The HNV F protein is a trimeric type I fusion protein that is initially expressed as an F precursor (F0), consisting of three domains (DI, DII and DIII), a C-terminal stem, a transmembrane domain and a cytoplasmic tail. We found that LayV F and MojV F both adopt a “tree-like” prefusion F structure similar to that of NiV, despite only sharing ~40% sequence conservation at the amino acid level. We show that despite sequence divergence from NiV, the F proteins adopt an overall similar structure but are antigenically distinct as they do not react to known antibodies or sera.

In August 2022, a novel henipavirus (HNV) named Langya virus (LayV) was isolated from patients with severe pneumonic disease in China. Based on the sequence of LayV, published in August 2022, we expressed the F ectodomain residues 1-478 without any heterologous stabilizing mutations. Through iterative particle picking, 2D classification and 3D refinements, we obtained a final structure of LayV F at 3.37 Å. In our analysis, we observed two particle populations that either had the stem domain displayed or not. Several rounds of heterogenous refinements and ab initio reconstructions using cryoSPARC were required to remove particles where the stem was not resolved. This yielded a final map including both the globular head domain and stem and resembled the “tree-like” conformation seen before for other HNV F proteins. LayV F DI is central to the monomer and is flanked by DII and DIII, the latter of which contains the fusion peptide (FP). Comparison of the trimers reveals a shift in the major outward facing DIII helix of LayV F relative to NiV, mediated by an adjacent loop region of a neighbouring protomer, which adopts an altered conformation in both MojV and LayV. The alternative cleavage site conformation for LayV is likely due to the presence of a bulkier hydrophobic leucine residue in position 413 in the adjacent DII (serine in the equivalent site in MojV), which would otherwise clash with the conserved and cleavage-site proximal tyrosine 102 (Y107 in MojV). In fact, our cryo-EM structure coupled with mass spectrometry analysis revealed that only positions N65 and N459 are glycosylated on LayV F, demonstrating that this glycoprotein is significantly less glycosylated in comparison to NiV.

>[3x]MAFLKSAIICYLLFYPHIVKSSLHYDSLSKVGIIKGLTYNYKIKGSPSTKLMVVKLIPNIDGVRNCTQKQFDEYKNLVKNVLEPVKLALNAMLDNVKSGNNKYRFAGAIMAGVALGVATAATVTAGIALHRSNENAQAIANMKNAIQNTNEAVKQLQLANKQTLAVIDTIRGEINNNIIPVINQLSCDTIGLSVGIKLTQYYSEILTAFGPALQNPVNTRITIQAISSVFNRNFDELLKIMGYTSGDLYEILHSGLIRGNIIDVDVEAGYIALEIEFPNLTLVPNAVVQELMPISYNVDGDEWVTLVPRFVLTRTTLLSNIDTSRCTVTESSVICDNDYALPMSYELIGCLQGDTSKCAREKVVSSYVPRFALSDGLVYANCLNTICRCMDTDTPISQSLGTTVSLLDNKKCLVYQVGDILISVGSYLGEGEYSADNVELGPPVVIDKIDIGNQLAGINQTLQNAEDYIEKSEEFLKG>MPLSAFSPPLPCDPARSHPTPEFPSSLQDYCEIRGIQSQPPARRDPTMDWLASLRSQIKPYRDRFPSHARLPRAGLPRAEILAEIAAMGAAESPAWRDGYASGAVYHGDEHHIAFLNEVYALQSQSNPLHPDLWPSTAKFEAEVVAMTAHMLGGDAAGGTVCGTVTSGGTESLLLAMKTYRDWARATKGITAPEAVVPVSAHAAFDKAAQYFGIKLVRTPLDADYRADVAAMREAITPNTVVVAGSAPGYPHGVVDPIPEIAALAAEHGIGCHVDACLGGFILPWAERLGYPVPPFDFRLEGVTSVSADTHKYGYGAKGTSVILYRRPDLLHYQYFIAADWPGGLYFSPTFAGSRPGALSATAWAAMLS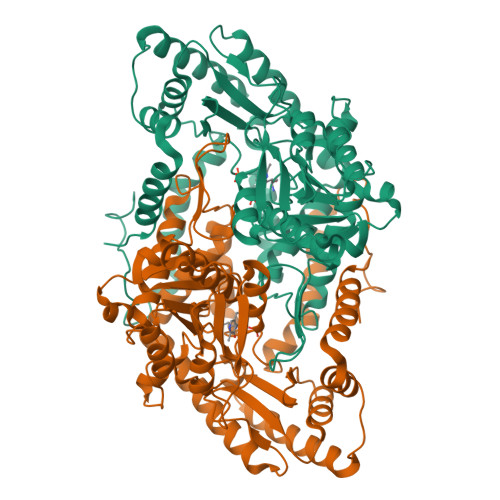LGEEGYLDATRRILQAADRLKAGVRAIPSLKILGDPLWVIAVASDELNIYQVMEEMAGRGWRLNGLHRPPAFHVALTLRHTEPGVVDRFLADLQDAVAQVRAHPEKATGMAPVYGMAAAAPPELVRQVLTGFIDLLYEVHHHHHH[2x]> MNSILGLIDTVTNTIGKAQQIELDKAALGQQRELALKRMKLDHQALNNQVEQFNKILEQRVQGPIQSVRLARAAGFRVDPYSYTDQNFYDDQ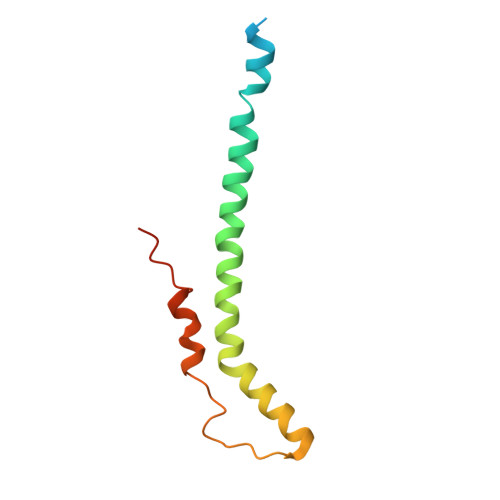LNAIRLSYRNLFKN>[4x]GVQLTAAQELMIQQLVAAQLQCNKRSFSDQPKVTPWPLGADPQSRDARQQRFAHFTELAIISVQEIVDFAKQVPGFLQLGREDQIALLKASTIEIMLLETARRYNHETECITFLKDFTYSKDDFHRAGLQVEFINPIFEFSRAMRRLGLDDAEYALLIAINIFSADRPNVQEPGRVEALQQPYVEALLSYTRIKRPQDQLRFPRMLMKLVSLRTLSSVHSEQVFALRLQDKKLPPLLSEIWDVHE

The liver X receptors (LXRs) alpha (LXRα, NR1H3) and beta (LXRβ, NR1H2) are members of the nuclear hormone receptor (NHR) superfamily of transcription factors that function as heterodimers with the retinoid X receptor (RXR) and activate or repress gene expression in response to binding of cholesterol derivatives or synthetic ligands. Transcriptional responses of LXRs are known to directly result from ligand-induced conformational changes in the receptor: similarly to other NHRs, in the absence of ligands or in the presence of antagonists, LXRs form complexes with corepressors, while binding of agonist ligands forces the C-terminal helix H12 of the receptor to fold into the active state that creates an activation function-2 (AF-2) coactivator-binding surface. Reaching isoform selectivity by rational structure-based drug design has proven to be difficult since the ligand-binding pockets (LBPs) of LXRα and LXRβ are virtually identical. Since the adverse lipogenic effects are considered to be largely driven by LXRα23,28, drug discovery efforts have focused on developing LXRβ-selective compounds.

In this study, we compared AZ876 with structurally related compounds AZ1–6. These compounds have a central cyclic sulfone amide scaffold with lipophilic substituents on both sides identical to AZ876, except for the tert-butyl substituent replaced by a propyl group in AZ1–3 and AZ6. The third substituent from the core is a larger elongated amine linker that is different in AZ1–6. The amine linker is mostly lipophilic with a polar group at the far end. The compounds AZ1, AZ3, and BMS-852927 have the highest affinities of 2, 4, and 3 nM, and the compounds AZ6, AZ7, and 24,25EC have the lowest affinities of 161, 105, and 133 nM, respectively. Analysis of crystal structures of LXRβ LBD in complex with WAY-254011, AZ3, AZ6, and AZ8, as well as of previously published crystal structures of LXRβ31,40,55 reveals that GW3965 and BMS-852927 are the only compounds not forming a direct hydrogen bond with LXRβ His435 and therefore they do not stabilize the His435–Trp457 activation switch crucial for the agonistic conformation of H12. Other agonists form shorter hydrogen bonds of 2.5–3.1 Å essential for proper position of H12, which correlates with their activities both in LXRβ HDX-MS and functional assays. Overall, most of the selected compounds displayed similar differential HDX patterns with a strong protection from deuterium exchange observed for the peptides lining the LBP: central part of H3, H5, β-sheet, and helices H6, H7, and H10/11.> MTLSIPPSIQCQTEAACRLITRVTGDTLRAIHLYGSAVAGGLKPNSDIDLLVTICQPLTEAQRATLMQELLALSSPPGASAEKRALEVTVVLYSQLVPWCFPPSREMQFGEWLREDICQGIYEPAQQDWDMVLLITQILETSIPLKGERAERLFTPAPAAQLLKALRYPLDLWQSTADVQGDEYHIVLTLARIWYTLSTGRFTSKDAAADWLLPQLPEDYAATLRAAQREYLGLEQQDWHILLPAVVRFVDFAKAHIPTQFTKG

Aminoglycoside resistance is commonly conferred by enzymatic modification of drugs by aminoglycoside-modifying enzymes such as aminoglycoside nucleo­tidyltransferases (ANTs). Still, the S. enterica genome contains an aadA gene encoding an ANT enzyme. AadA is an ANT(3′′)(9) streptomycin/spectinomycin adenyltransferase encoded by the aadA gene that adenylates the 3′′-hydroxyl group of the streptomycin glucosamine ring and the 9-hydroxyl group of the spectinomycin actinamine ring. AadA catalyses the magnesium-dependent transfer of adenosine monophosphate from ATP to the two chemically dissimilar drugs streptomycin and spectinomycin. AadA consists of a nucleotidyltransferase domain and an α-helical bundle domain.

Here, the first crystal structure of an ANT(3′′)(9) adenyltransferase, AadA from Salmonella enterica, is presented. Trials to perform molecular replacement using search models with low sequence identity failed, and the structure was solved using SAD phasing with selenomethionine-substituted AadA crystals. The final model contains residues 3–262 and only lacks the first two N-terminal residues and the His tag. The loop regions 97–103 and 235–240 display weak density, indicating flexibility. The N-terminal domain (residues 3–157) forms a nucleotidyltransferase fold according to the SCOP database and has a central five-stranded mixed β-sheet surrounded by six α-helices. The C-terminal domain (residues 158–262) consists of five α-helices forming an up-and-down α-helical bundle. AadA crystallizes as a monomer and is a monomer in solution as confirmed by small-angle X-ray scattering, in contrast to structurally similar homodimeric adenylating enzymes such as kanamycin nucleotidyltransferase. In the AadA structure, several of the residues predicted to participate in ATP binding are involved in interactions with the C-terminal domain: Ser36 forms a hydrogen bond to Asp206, Ser46 hydrogen-bonds to the amino group of Lys43, and Asp47 and Asp49 form salt bridges with Lys205. Thus, in the conformation observed in the apo AadA structure the nucleotide-binding site is blocked by interdomain inter­actions.>[2x]GGSRCQRDHLSTKLIPTEVPADLIRAVTCQVCDHLLSDPVQSPCRHLFCRLCIIRYTHALGPNCPTCNQHLNPSHLIKPAKFFLATLSSLPLLCPSEECSDWVRLDSFREHCLNHYREKESQEEQTPSEQNLDGYLPVNKGGRPRQHLLSLTRRAQKHRLRDLKNQVKTFAE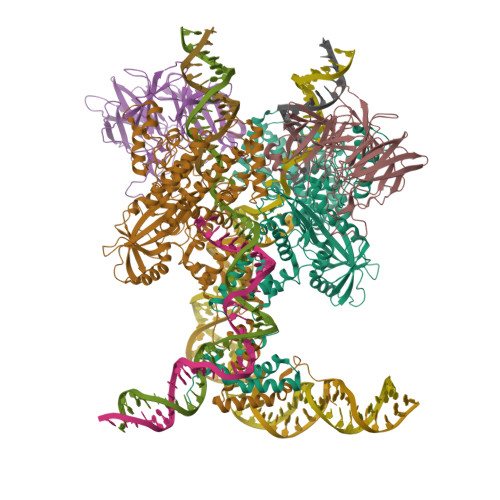KEEGGDVKSVCLTLFLLALRAGNEHKQADELEAMMQGRGFGLHPAVCLAIRVNTFLSCSQYHKMYRTVKATSGRQIFQPLHTLRNAEKELLPGFHQFEWQPALKNVSTSWDVGIIDGLSGWTVSVDDVPADTISRRFRYDVALVSALKDLEEDIMEGLRERALDDSMCTSGFTVVVKESCDGMGDVSEKHGSGPAVPEKAVRFSFTIMSISIRLEGEDDGITIFQEQKPNSELSCRPLCLMFVDESDHETLTAILGPVVAERKAMMESRLIISVGGLLRSFRFFFRGTGYDEKMVREMEGLEASGSTYICTLCDSTRAEASQNMVLHSITRSHDENLERYEIWRKNPFSESADELRDRVKGVSAKPFMETQPTLDALHCDIGNATEFYKIFQDEIGEVYQKPNPSREERRRWRSTLDKQLRKKMKLKPVMRMNGNYARRLMTREAVEAVCELVPSEERREALLKLMDLYLQMKPVWRSTCPSRDCPDQLCQYSYNSQQFADLLSSMFKYRYDGKITNYLHKTLAHVPEIVERDGSIGAWASEGNESGNKLFRRFRKMNARQSKTFELEDILKHHWLYTSKYLQKFMEAHKNS;>GGSMSLQPLTAVNCGSLVQPGFSLLDLEGDVYLFGQKGWPKRSCPTGIFGVRIKKGELKLRAISFSNNSSYLPPLRCPAIAHFEAQDGKPECYLIHGGRTPNNELSSSLYMLSVDSRGCNRKVTLRCEEKELVGDVPSARYGHTLSVINSRGKTACVLFGGRSYMPPTERTTQNWNSVVDCPPQVYLIDLEFGCCTAHTLPELTDGQSFHVALARQDCVYFLGGHILSSDCRPSRLIRLHVELLLGSPVLTCTILHEGLTITSAIASPIGYHEYIIFGGYQSETQKRMECTYVGLDDVGVHMESREPPQWTSEISHSRTWFGGSLGKGTALVAIPSEGNPTPPEAYHFYQVSFQKEQDGEATAQGGSQESTDFEDSAPLEDSEELYFGREPHELEYSSDVEGDTYNEEDEEDESQTGYWIKCCLSCQVDPNIWEPYYSTELTRPAMIFCSRGEGGHWVHAQCMELPESLLLQLSQDNSKYFCLDHGGLPKQEMTPPKQMLPVKRVPMKMTHRKAPVSLKMTPAKKTFLRRLFD[2x]>[2x]LVSKLSQLQTELLAALLESALSKEAL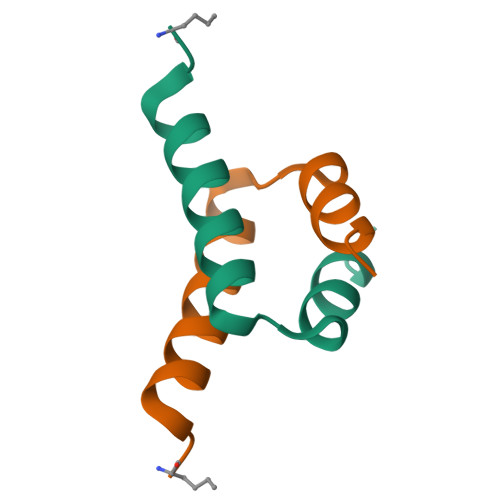IQALGEW>[2x]MQGSVTEFLKPRLVDIEQVSSTHAKVTLEPLERGFGHTLGNALRRILLSSMPGCAVTEVEIDGVLHEYSTKEGVQEDILEILLNLKGLAVRVQGKDEVILTLNKSGIGPVTAADITHDGDVEIVKPQHVICHLTDENASISMRIKVQRGRGYVPASTRIHSEEDERPIGRLLVDACYSPVERIAYNVEAARVEQRTDLDKLVIEMETNGTIDPEEAIRRAATILAEQLEAFVDLEVLFQ;> MVYSYTEKKRIRKDFGKRPQVLDVPYLLSIQLDSFQKFIEQDPEGQYGLEAAFRSVFPIQSYSGNSELQYVSYRLGEPVFDVQECQIRGVTYSA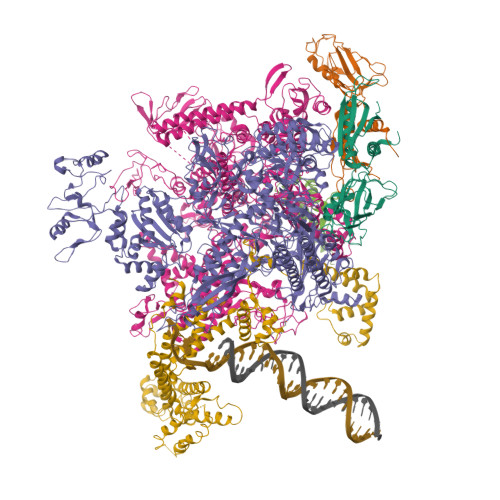PLRVKLRLVIYEREAPEGTVKDIKEQEVYMGEIPLMTDNGTFVINGTERVIVSQLHRSPGVFFDSDKGKTHSSGKVLYNARIIPYRGSWLDFEFDPKDNLFVRIDRRRKLPATIILRALNYTTEQILDLFFEKVIFEIRDNKLQMELVPERLRGETASFDIEANGKVYVEKGRRITARHIRQLEKDDVKLIEVPVEYIAGKVVAKDYIDESTGELICAANMELSLDLLAKLSQSGHKRIETLFTNDLDHGPYISETLRVDPTNDRLSALVEIYRMMRPGEPPTREAAESLFENLFFSEDRYDLSAVGRMKFNRSLLREEIEGSGILSKDDIIDVMKKLIDIRNGKGEVDDIDHLGNRRIRSVGEMAENQFRVGLVRVERAVKERLSLGDLDTLMPQDMINAKPISAAVKEFFGSSQLSQFMDQNNPLSEITHKRRISALGPGGLTRERAGFEVRDVHPTHYGRVCPIETPEGPNIGLINSLSVYAQTNEYGFLETPYRKVTDGVVTDEIHYLSAIEEGNYVIAQANSNLDEEGHFVEDLVTCRSKGESSLFSRDQVDYMDVSTQQVVSVGASLIPFLEHDDANRALMGANMQRQAVPTLRADKPLVGTGMERAVAVDSGVTAVAKRGGVVQYVDASRIVIKVNEDEMYPGEAGIDIYNLTKYTRSNQNTCINQMPCVSLGEPVERGDVLADGPSTDLGELALGQNMRVAFMPWNGYNFEDSILVSERVVQEDRFTTIHIQELACVSRDTKLGPEEITADIPNVGEAALSKLDESGIVYIGAEVTGGDILVGKVTPKGETQLTPEEKLLRAIFGEKASDVKDSSLRVPNGVSGTVIDVQVFTRDGVEKDKRALEIEEMQLKQAKKDLSEELQILEAGLFSRIRAVLVAGGVEAEKLDKLPRDRWLELGLTDEEKQNQLEQLAEQYDELKHEFEKKLEAKRRKITQGDDLAPGVLKIVKVYLAVKRRIQPGDKMAGRHGNKGVISKINPIEDMPYDENGTPVDIVLNPLGVPSRMNIGQILETHLGMAAKGIGDKINAMLKQQQEVAKLREFIQRAYDLGADVRQKVDLSTFSDEEVMRLAENLRKGMPIATPVFDGAKEAEIKELLKLGDLPTSGQIRLYDGRTGEQFERPVTVGYMYMLKLNHLVDDKMHARSTGSYSLVTQQPLGGKAQFGGQRFGEMEVWALEAYGAAYTLQEMLTVKSDDVNGRTKMYKNIVDGNHQMEPGMPESFNVLLKEIRSLGINIELEDE;> VKDLLKFLKAQTKTEEFDAIKIALASPDMIRSWSFGEVKKPETINYRTFKPERDGLFCARIFGPVKDYECLCGKYKRLKHRGVICEKCGVEVTQTKVRRERMGHIELASPTAHIWFLKSLPSRIGLLLDMPLRDIERVLYFESYVVIEGGMTNLERQQILTEEQYLDALEEFGDEFDAKMGAEAIQALLKSMDLEQECEQLREELNETNSETKRKKLTKRIKLLEAFVQSGNKPEWMILTVLPVLPPDLRPLVPLDGGRFATSDLNDLYRRVINRNNRLKRLLDLAAPDIIVRNEKRMLQEAVDALLDNGRRGRAITGSNKRPLKSLADMIKGKQGRFRQNLLGKRVDYSGRSVITVGPYLRLHQCGLPKKMALELFKPFIYGKLELRGLATTIKAAKKMVEREEAVVWDILDEVIREHPVLLNRAPTLHRLGIQAFEPVLIEGKAIQLHPLVCAAYNADFDGDQMAVHVPLTLEAQLEARALMMSTNNILSPANGEPIIVPSQDVVLGLYYMTRDCVNAKGEGMVLTGPKEAERLYRSGLASLHARVKVRITEYEKDANGELVAKTSLKDTTVGRAILWMIVPKGLPYSIVNQALGKKAISKMLNTCYRILGLKPTVIFADQIMYTGFAYAARSGASVGIDDMVIPEKKHEIISEAEAEVAEIQEQFQSGLVTAGERYNKVIDIWAAANDRVSKAMMDNLQTETVINRDGQEEKQVSFNSIYMMADSGARGSAAQIRQLAGMRGLMAKPDGSIIETPITANFREGLNVLQYFISTHGARKGLADTALKTANSGYLTRRLVDVAQDLVVTEDDCGTHEGIMMTPVIEGGDVKEPLRDRVLGRVTAEDVLKPGTADILVPRNTLLHEQWCDLLEENSVDAVKVRSVVSCDTDFGVCAHCYGRDLARGHIINKGEAIGVIAAQSIGEPGTQLTMRTFHIGGAASRAAAESSIQVKNKGSIKLSNVKSVVNSSGKLVITSRNTELKLIDEFGRTKESYKVPYGAVLAKGDGEQVAGGETVANWDPHTMPVITEVSGFVRFTDMIDGQTITRQTDELTGLSSLVVLDSAERTAGGKDLRPALKIVDAQGNDVLIPGTDMPAQYFLPGKAIVQLEDGVQISSGDTLARIPQESGGTKDITGGLPRVADLFEARRPKEPAILAEISGIVSFGKETKGKRRLVITPVDGSDPYEEMIPKWRQLNVFEGERVERGDVISDGPEAPHDILRLRGVHAVTRYIVNEVQDVYRLQGVKINDKHIEVIVRQMLRKATIVNAGSSDFLEGEQVEYSRVKIANRELEANGKVGATYSRDLLGITKASLATESFISAASFQETTRVLTEAAVAGKRDELRGLKENVIVGRLIPAGTGYAYHQDRMRRRAAGEAPAAPQVTAEDASASLAELLNAGLGGSDNELE;> MARVTVQDAVEKIGNRFDLVLVAARRARQMQVGGKDPLVPEENDKTTVIALREIEEGLINNQILDVRERQEQQEQEAAELQAVTAIAEGRR;> MEQNPQSQLKLLVTRGKEQGYLTYAEVNDHLPEDIVDSDQIEDIIQMINDMGIQVMEEAPDADDLMLAENTADEDAAEAAAQVLSSVESEIGRTTDPVRMYMREMGTVELLTREGEIDIAKRIEDGINQVQCSVAEYPEAITYLLEQYNRVEAEEARLSDLITGFVDPNAEEDLAPTATHVGSELSQEDLDDDEDEDEEDGDDDSADDDNSIDPELAREKFAELRAQYVVTRDTIKAKGRSHATAQEEILKLSEVFKQFRLVPKQFDYLVNSMRVMMDRVRTQERLIMKLCVEQCKMPKKNFITLFTGNETSDTWFNAAIAMNKPWSEKLHDVSEEVHRALQKLQQIEEETGLTIEQVKDINRRMSIGEAKARRAKKEMVEANLRLVISIAKKYTNRGLQFLDLIQEGNIGLMKAVDKFEYRRGYKFSTYATWWIRQAITRSIADQARTIRIPVHMIETINKLNRISRQMLQEMGREPTPEELAERMLMPEDKIRKVLKIAKEPISMETPIGDDEDSHLGDFIEDTTLELPLDSATTESLRAATHDVLAGLTAREAKVLRMRFGIDMNTDYTLEEVGKQFDVTRERIRQIEAKALRKLRHPSRSEVLRSFLDD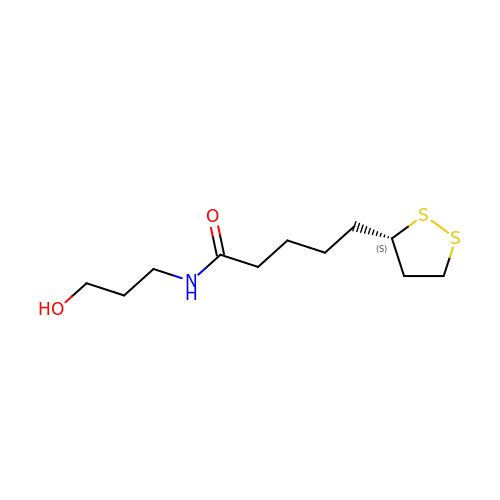5-[(3~{S})-1,2-dithiolan-3-yl]-~{N}-(3-oxidanylpropyl)pentanamide | C11 H21 N O2 S2 | QPQPASXMSHOHIW-JTQLQIEISA-N> ADCSSDLTSGISTKRIYYVAPNGNSSNNGSSFNAPMSFSAAMAAVNPGELILLKPGTYTIPYTQGKGNTITFNKSGKDGAPIYVAAANCGRAVFDFSFPDSQWVQASYGFYVTGDYWYFKGVEVTRAGYQGAYVIGSHNTFENTAFHHNRNTGLEINNGGSYNTVINSDAYRNYDPKKNGSMADGFGPKQKQGPGNRFVGCRAWENSDDGFDLFDSPQKVVIENSWAFRNGINYWNDSAFAGNGNGFKLGGNQAVGNHRITRSVAFGNVSKGFDQNNNAGGVTVINNTSYKNGINYGFGSNVQSGQKHYFRNNVSLSASVTVSNADAKSNSWDTGPAASASDFVSLDTSLATVSRDNDGTLPETSLFRLSAN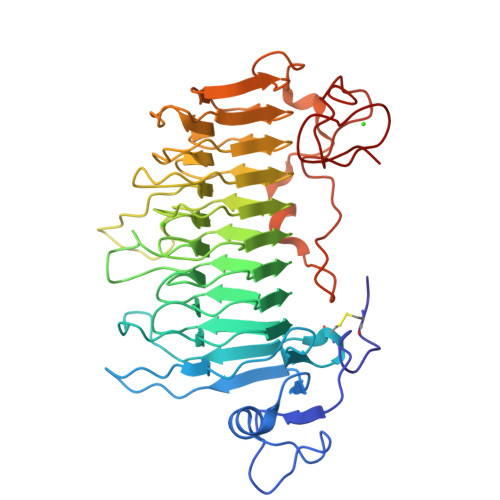SKLINAGTKESNISYSGSAPDLGAFERN4-(ethylsulfanyl)benzoic 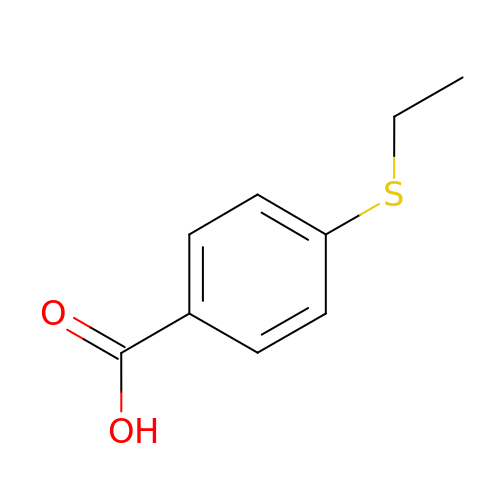acid | C9 H10 O2 S | LDYCQBKCUOVGDA-UHFFFAOYSA-N>[2x]MLKNVLRYPGGKSKALKYILPNLPVGFREYREPMVGGGAVALAVKQLYTNVKIKINDLNYDLICFWKQLRDNPVQLIEEVSKIKENYKDGRKLYEFLTSQNGGGEFERAVR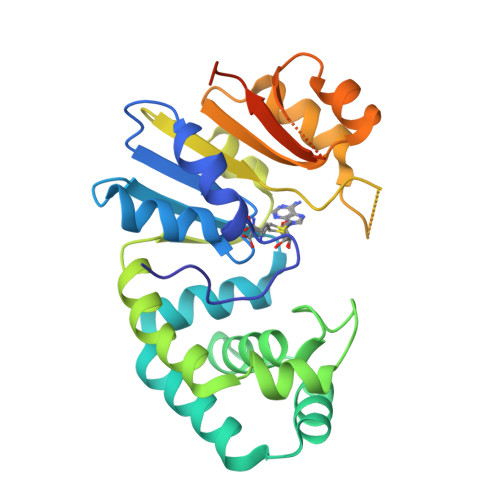FYILNRITFSGTVDSGGYSQQSFENRFTWSAINKLKQAAEIIKDFEISHGDYEKLLFEPGNEVFIFLDPPYYSTTESRLYGKNGDLHLSFDHERFAFNIKKCPHLWMITYDDSPEVRKLFKFANIYEWELQYGMNNYKQSKAEKGKELFITNYKLEELRQKEKYALGLLEHHHHHH N-{4-[4-AMINO-6-(4-METHOXYPHENYL)FURO[2,3-D]PYRIMIDIN-5-YL]PHENYL}-N'-[2-FLUORO-5-(TRIFLUOROMETHYL)PHENYL]UREA 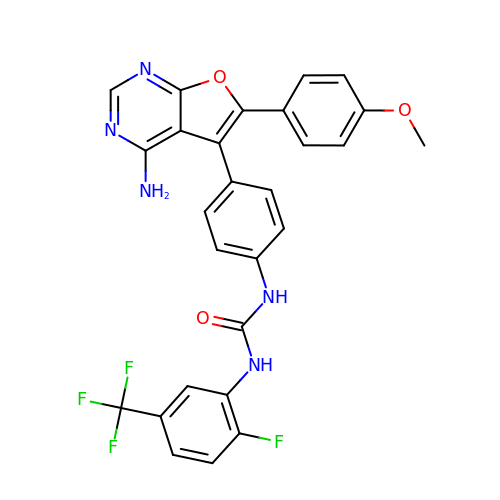| C27 H19 F4 N5 O3 | FGZIONRFHVNRJB-UHFFFAOYSA-N>[3x]MGSSHHHHHHSMDNKTE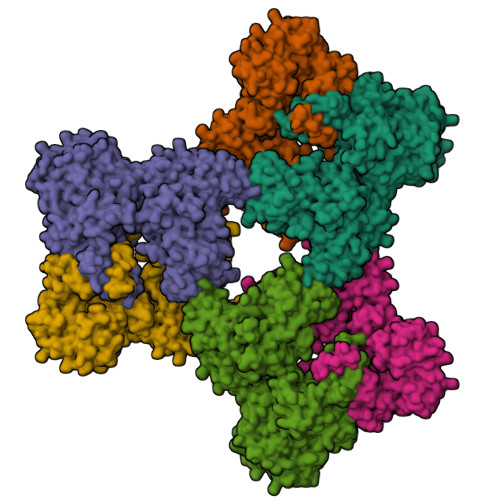TKIEPKTGTTNFDQEALLYHQQGKPGKIEVISSKPCATEKDLSLAYSPGVAAPCKAIAKDPAKVYDYTAKGNLVAVISNGTAVLGLGNIGPAAGKPVMEGKGILFKQFAGIDVFDIEVAATDVDVFCNAVRVLEPTFGGINLEDIKAPECFEIEERLKKEMNIPVFHDDQHGTAIVSGAALLNACSITNRKMETVRIVVNGAGASANSCAKIFIALGARRENIIMCDSQGVIYKGRTAGMNKYKEYFASETEARTLTEALRGADVFVGLSVAGALTPEMLKDMAKDPIIFAMANPEPEITPDKARAARPDAIIATGRSDYPNQVNNVLGFPSIFRGALDTRSTQINEEMKLAAVHALAKLAREDVPDKVSATYGGKSFKFGRDYLIPKPFDTRVLLWVAPEVAKAAMKSGVATRAIEDWDQYRESLEALQGPSKVFIRSAINRVHQNSAANGGELPRIVFPEGTSTKVLKALATLVEEKICQPILLGYPERVKEKIKALDIPLLNDVSIVHPSSHPKYFSFVEKLYSLRQRKGINLGEAERLMADPNYFAAMMVNQGEADGMVSGSSINYADAVRPILQTIGVYKEGIPAGLNFVLLEDKFLVLADTTVNLNPTAEQCAQIALQAAKIVEYFGIEPRVAMLSYSNFSGAEGTPRKMKKAAEIARSLRPDLMIEGDMQADTAVNPEIMERLFPFSGLKGGANVLVFPNLESSNIAYKLIQQIGKAEVIGPFLTGVRRSANVLQRTTTVDGIVNSVVFTALEAQYIKEVLKSRGKK> MENKNGGYLPEEEIPDQPPATGAFNYGEALQKAIFFYECQRSGKLDSSTLRLNWRGDSGLDDGKDAGIDLTGGWYDAGDHVKFNLPMSYSAAMLGWAVYEYEDAFKQSGQYNHILNNIKWACDYFIKCHPEKDVYYYQVGDGHADHAWWGPAEVMPMERPSYKVDRSSPGSTVVAETSAALAIASIIFKKVDGEYSKECLKHAKELFEFADTTKSDDGYTAANGFYNSWSGFYDELSWAAVWLYLATNDSSYLDKAESYSDKWGYEPQTNIPKYKWAQCWDDVTYGTYLLLARIKNDNGKYKEAIERHLDWWTTGYNGERITYTPKGLAWLDQWGSLRYATTTAFLACVYSDWENGDKEKAKTYLEFARSQADYALGSTGRSFVVGFGENPPKRPHHRTAHGSWADSQMEPPEHRHVLYGALVGGPDSTDNYTDDISNYTCNEVACDYNAGFVGLLAKMYKLYGEL;> MGSPDPKFNGIEEVPEDEIFVEAGVNASGNNFIEIKAIVNNKSGWPARVCENLSFRYFINIEEIVNAGKSASDLQVSSSYNQGAKLSDVKHYKDNIYYVEVDLSGTKIYPGGQSAYKKEVQFRISAPEGTVFNPENDYSYQGLSAGTVVKSEYIPVYDA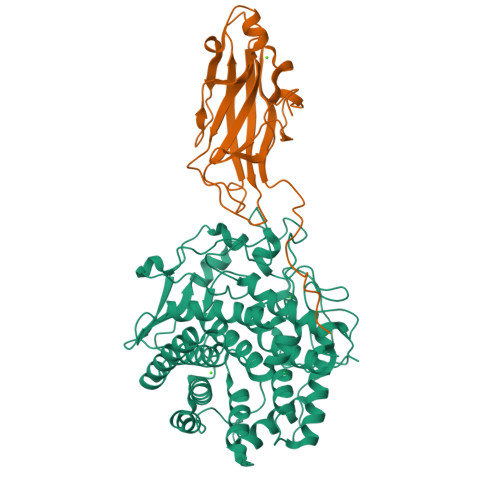GVLVFGREPLEHHHHHH>AIKLEHEIKVTDQALFFDGVKKSVPQARTQAYIEGQKYNYAYGNAIAPHGDAIKVYKNYVFMTWYRGGILDRHVMLTRYNTLTGKSVTIEFPHQHTGFEGRWWVGETHNTIAVAISPKDETIHLLYDMHAYRENTDTGGNGDIRKDYFRYSYSLAGAASVTDNNFTLTQFVKDTSVNSEGATDYKHLTMTGIEDHGQFSRLTYPTFFTSHDGDLFLHMRQGSSHDGRVVFNKYLAEQGKWSHFKSFNVLGAGKKGEIKNWSIYGKMKYADGKIRIGFQRRFNLPDRFRAQDGMFYAYSDDPSGETQWKNYKGEAITMPLVKADEALVMRPGDLLPDATAKDQVSITGGFDWTVTENGDLHLIGQTNEWVNKKVIKK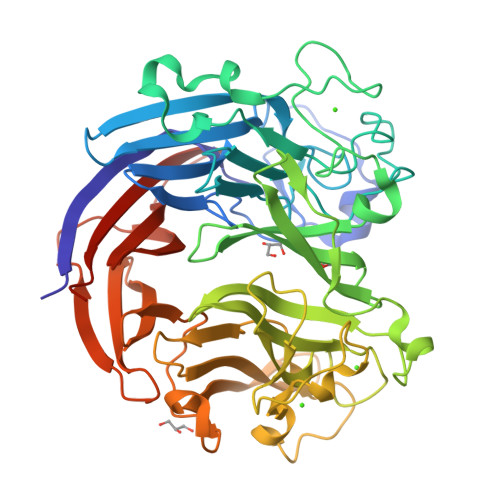VYSHTYQKAGVGELITTTDFPPASQLYTAGENIYIIGLEQGRPFVEQAKGGTNDFTRVYYAPVGSQSFQKGIVHIHDGKLYYYLLEKGGAGDKRTTYLQIINLDIDSKSYFKKIKQ[2x]>GKKVLIVYAHQEPKSFNGSLKNVAVDELSRQGCTVTVSDLYAMNFEPRATDKDITGTLSNPEVFNYGVETHEAYKQRSLASDITDEQKKVREADLVIFQFPLYWFSVPAILKGWMDRVLCQGFAFDIPGFYDSGLLQGKLALLSVTTGGTAEMYTKTGVNG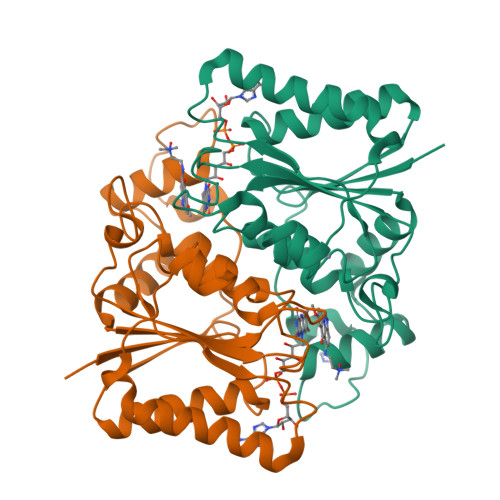DSRYFLWPLQHGTLHFCGFKVLAPQISFAPEIASEEERKGMVAAWSQRLQTIWKEEPIPCTAHWHFG[2x]> MAHAGGGSGGSGAGGPAGRGLSGARWGRSGSAGHEKLPVHVEDALTYLDQVKIRFGSDPATYNGFLEIMKEFKSQSIDTPGVIRRVSQLFHEHPDLIVGFNAFLPLGYRIDIPKNGKLNIQSPLTSQENSHNHGDGAEDFKQQVPYKEDKPQVPLESDSVEFNNAISYVNKIKTRFLDHPEIYRSFLEILHTYQKEQLNTRGRPFRGMSEEEVFTEVANLFRGQEDLLSEFGQFLPEAKRSLFTGNGPCEMHSVQKNEHDKTPEHSRKRSRPSLLRPVSAPAKKKMKLRGTKDLSIAAVGKYGTLQEFSFFDKVRRVLKSQEVYENFLRCIALFNQELVSGSELLQLVSPFLGKFPELFAQFKSFLGVKELSFAPPMSDRSGDGISREIDYASCKRIGSSYRALPKTYQQPKCSGRTAICKEVLNDTWVSFPSWSEDSTFVSSKKTPYEEQLHRCEDERFELDVVLETNLATIRVLESVQKKLSRMAPEDQEKFRLDDSLGGTSEVIQRRAIYRIYGDKAPEIIESLKKNPVTAVPVVLKRLKAKEEEWREAQQGFNKIWREQYEKAYLKSLDHQAVNFKQNDTKALRSKSLLNEIESVYDEHQEQHSEGRSAPSSEPHLIFVYEDRQILEDAAALISYYVKRQPAIQKEDQGTIHQLLHQFVPSLFFSQQLDLGASEESADEDRDSPQGQTTDPSERKKPAPGPHSSPPEEKGAFGDAPATEQPPLPPPAPHKPLDDVYSLFFANNNWYFFLRLHQTLCSRLLKIYRQAQKQLLEYRTEKEREKLLCEGRREKGSDPAMELRLKQPSEVELEEYYPAFLDMVRSLLEGSIDPTQYEDTLREMFTIHAYVGFTMDKLVQNIARQLHHLVSDDVCLKVVELYLNEKKRGAAGGNLSSRCVRAARETSYQWKAERCMADENCFKVMFLQRKGQVIMTIELLDTEEAQTEDPVEVQHLARYVEQYVGTEGASSSPTEGFLLKPVFLQRNLKKFRRRWQSEQARALRGEARSSWKRLVGVESACDVDCRFKLSTHKMVFIVNSEDYMYRRGTLCRAKQVQPLVLLRHHQHFEEWHSRWLEDNVTVEAASLVQDWLMGEEDEDMVPCKTLCETVHVHGLPVTRYRVQYSRRPASP;> MAYSQGGGKKKVCYYYDGDIGNYYYGQGHPMKPHRIRMTHNLLLNYGLYRKMEIYRPHKATAEEMTKYHSDEYIKFLRSIRPDNMSEYSKQMQRFNVGEDCPVFDGLFEFCQLSTGGSVAGAVKLNRQQTDMAVNWAGGLHHAKKSEASGFCYVNDIVLAILELLKYHQRVLYIDIDIHHGDGVEEAFYTTDRVMTVSFHKYGEYFPGTGDLRDIGAGKGKYYAVNFPMRDGIDDESYGQIFKPIISKVMEMYQPSAVVLQCGADSLSGDRLGCFNLTVKGHAKCVEVVKTFNLPLLMLGGGGYTIRNVARCWTYETAVALDCEIPNELPYNDYFEYFGPDFKLHISPSNMTNQNTPEYMEKIKQRLFENLRMLPHAPGVQMQAIPEDAVHEDSGDEDGEDPDKRISIRASDKRIACDEEFSDSEDEGEGGRRNVADHKKGAKKARIEEDKKETEDKKTDVKEEDKSKDNSGEKTDTKGTKSEQLSNP;> MWEKMETKTIVYDLDTSGGLMEQIQALLAPPKTDEAEKRSRKPEKEPRRSGRATNHDSCDSCKEGGDLLCCDHCPAAFHLQCCNPPLSEEMLPPGEWMCHRCTVRRKKREQKKELGHVNGLVDKSGKRTTSPSSDTDLLDRSASKTELKAIAHARILERRASRPGTPTSSASTETPTSEQNDVDEDIIDVDEEPVAAEPDYVQPQLRRPFELLIAAAMERNPTQFQLPNELTCTTALPGSSKRRRKEETTGKNVKKTQHELDHNGLVPLPVKVCFTCNRSCRVAPLIQCDYCPLLFHMDCLEPPLTAMPLGRWMCPNHIEHVVLNQKNMTLSNRCQVFDRFQDTVSQHVVKVDFLNRIHKKHPP

Histone deacetylase complexes remove histone acetylation, thereby repressing transcription and regulating the transcriptional output of each gene. In order to address this, we reconstituted a recombinant version of the human SIN3B complex, composed of the subunits SIN3B isoform 2, HDAC2 (hereafter named HDAC for simplicity), PHF12 and MORF4L1, expressed in the baculovirus/insect cell system. Remarkably, SIN3B encircles the deacetylase and contacts its allosteric basic patch thereby stimulating catalysis. A SIN3B loop inserts into the catalytic tunnel, rearranges to accommodate the acetyl-lysine moiety, and stabilises the substrate for specific deacetylation, which is guided by a substrate receptor subunit.

Moreover, we obtained an additional map of the catalytic SIN3B core subcomplex (SIN3Bcore) at the resolution of 2.8 Å. SIN3Bcore cryo-EM density map at 2.8 Å resolution is shown for relevant sidechains and water molecules. As detailed above, our cryo-EM structure of the SIN3B complex shows that a loop connecting MD and HID domains (Gate loop) inserts into the active site of the enzyme. SIN3B Glu436 enters the active site and its carboxyl group establishes hydrogen bonds with the catalytic HDAC His179, whereas the Cβ and Cγ of Glu436 makes non-polar contacts with HDAC Phe206. The Cβ of the following SIN3B Asp437 makes non-polar contacts with the HDAC hydrophobic Leu272 and Pro30. 16, we could also find an acetate molecule coordinating with the catalytic zinc cation and the catalytic Tyr304. This suggests that our SIN3B apo structure represents a post-hydrolysis state of the deacetylation reaction where the protein substrate has been released and the gate loop has returned to a conformation in which it occludes the active site. Strikingly, in our structure the SIN3B HID domain binds directly the allosteric basic patch of HDAC, preventing InsP binding. This interaction is dominated by a triad of SIN3B acidic residues coming from the stalk region of the HID i.e., Glu456, Asp457 and Glu461. Specifically, Glu456 and Asp457 interact with HDAC Lys32 and Arg271 via a network of hydrogen bonds involving water molecules.>[4x]MSVNNPQTREWQTLSGEHHLAPFSDYKQLKEKGPRIITKAQGVHLWDSEGHKILDGMAGLWCVAVGYGREELVQAAEKQMRELPYYNLFFQTAHPPALELAKAITDVAPKGMTHVFFTGSGSEGNDTVLRMVRHYWALKGKPHKQTIIGRINGYHGSTFAGACLGGMSGMHEQGGLPIPGIVHIPQPYWFGEGGDMTPDEFGVWAAEQLEKKILEVGEDNVAAFIAEPIQGAGGVIIPPETYWPKVKEILARYDILFVADEVICGFGRTGEWFGSDYYDLKPDLMTIAKGLTSGYIPMGGVIVRDTVAKVISEGGDFNHGFTYSGHPVAAAVGLENLRILRDEKIVEKARTEAAPYLQKRLRELQDHPLVGEVRGLGMLGAIELVKDKATRSRYEGKGVGMICRTFCFENGLIMRAVGDTMIIAPPLVISHAEIDELVEKARKCLDLTLEAIQ

Omega transaminases (ω-TAs) can mediate the chiral amination of several unnatural substrates without the requirement of an α-COOH group and are highly relevant in the production of several pharmaceutical intermediates of commercial interest. In this work, we successfully overexpressed and characterized the two recombinant transaminases TA_2799 and TA_5182 from P. putida KT2440 and solved their crystal structures. The overall structural fold of the TA_5182 and TA_2799 enzymes is similar to that observed for other class III fold type I TAs with two α/β domains. There are two highly flexible loops present in the structures of TA_2799 and TA_5182 that mediate the entry and exit of the cofactor and the substrate/byproduct into the active site of the enzyme, leading to significant conformational changes in the enzyme structure.

We determined the structure of TA_5182 in both relaxed (open) and closed states, mimicking the cofactor-free and the cofactor-bound form of the enzyme, respectively. The open state of TA_5182 is not easily observed. It shows a distinct conformation in the overall ternary structure of the enzyme, which allows the cofactor molecule and the substrates to enter the enzyme’s active site via movement of the flexible loops. In the crystal structure of the open state of TA_5182, these residues could not be built due to poor electron density in this region and hence were excluded from the final refined model. In the crystal structure of the open state of TA_5182, the “lid” loop could not be visualized due to the inherent flexibility of this region. In our crystal structure of the apo state of TA_5182, the electron density of the roof loop is visible. Comparing the open state of TA_5182 with the deposited structures in PDB resulted in an average RMSD of 2.0 Å, which is expected as the conformation of this state is significantly different than the PLP-bound state of the enzyme. The major conformational differences can be found in the roof loop and the outer loop in the open state of TA_5182. In the apo-open state, the F321 in TA_5182 is initially positioned near the surface of the enzyme, widening the substrate entry channel of the enzyme. Y322 is initially in a hydrogen bond with T127.(3~{S})-3-methyl-2-oxidanylidene-pentanedioic acid | C6 H8 O5 | 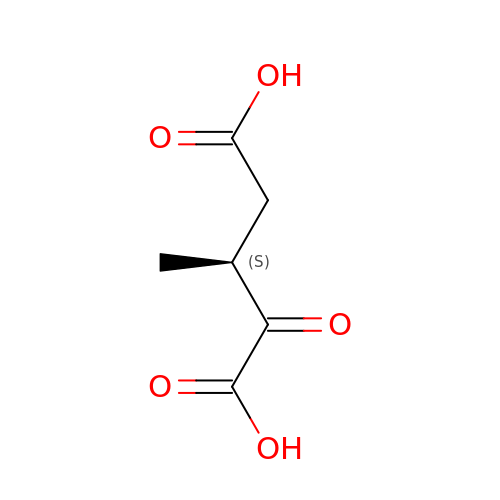BJQIUPTURRAODO-VKHMYHEASA-N> GNKWNTTLPGGNMQFQGVIIAETCRIEAGDKQMTVNMGQISSNRFHAVGEDSAPVPFVIHLRECSTVVSERVGVAFHGVADGKNPDV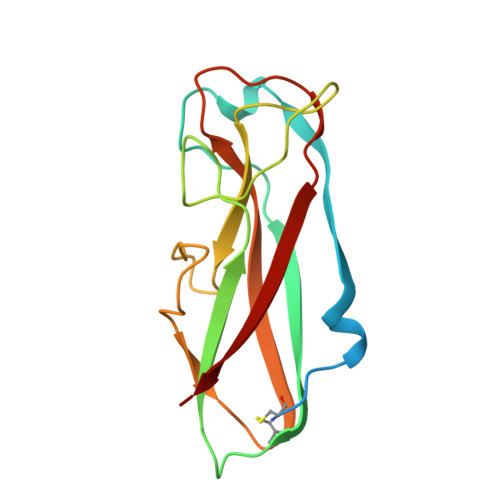LSVGEGPGIATNIGVALFDDEGNLVPINRPPANWKRLYSGSTSLHFIAKYRATGRRVTGGIANAQAWFSLTYQ> MSVIQNYNKALQQLEKYKPYEEALLQAEAPRLAEYQAYIDFEMKIGDPARIQLIFER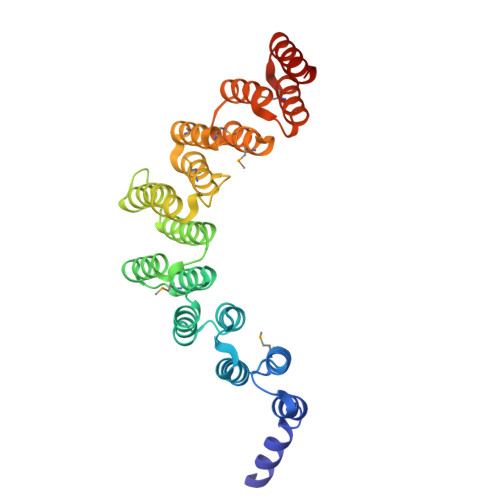ALVENCLVPDLWIRYSQYLDRQLKVKDLVLSVHNRAIRNCPWTVALWSRYLLAMERHGVDHQVISVTFEKALNAGFIQATDYVEIWQAYLDYLRRRVDFKQDSSKELEELRAAFTRALEYLKQEVEERFNESGDPSCVIMQNWARIEARLCNNMQKARELWDSIMTRGNAKYANMWLEYYNLERAHGDTQHCRKALHRAVQCTSDYPEHVCEVLLTMERTEGSLEDWDIAVQKTETRLARVNE Wzc, an integral cytoplasmic membrane tyrosine autokinase protein serves as the master regulator of the biosynthesis and export of many bacterial capsular polysaccharides and exopolysaccharides. Wzc comprises a large periplasmic domain, two transmembrane helices and a C-terminal cytoplasmic kinase domain with a tyrosine-rich tail. Wzc regulates polymerisation functions through cycling the formation and dissociation of an octameric complex, driven by changes in the phosphorylation status of the tyrosine-rich tail. E. coli Wzc serves a model for a wider family of polysaccharide co-polymerases.

Here, we report the characterisation of the structures WzcK540M2YE (Y718E, Y717E), WzcK540M3YE (Y718E, Y717E and Y715E) and WzcK540M3YE_N711Y (an additional N711Y mutation) corresponding to different phosphorylation states. When Y715 occupies the active site (1pY), Y713 is bound in the same pocket. The structural and MD data reported here confirm this hypothesis, showing that the tyrosine most stably positioned at the active site is the one immediately N-terminal to the phosphotyrosine (or the engineered Tyr-to-Glu mutation). We show that it is binding of the i-2 tyrosine to the tyrosine pocket (where i is the number of the residue positioned at the kinase active site) orders the tail between the tyrosine at the active site and helix α23. The presence of the negatively charged E675 in the tyrosine pocket we suggest is incompatible with binding a negatively charged phosphorylated tyrosine (or glutamic acid side chain). During the progressive phosphorylation sequence, the kinase domain is a rigid body. Structural alignment of the kinase domains of monomers of the full-length protein reveals increasing tilting of the transmembrane and periplasmic regions. When the octamer is viewed from the periplasm to the cytoplasm, progressive phosphorylation results in a clockwise rotation of transmembrane and periplasmic regions relative to the kinase ring. The movement of helix α1 is directly transmitted to transmembrane helix α2 and then to the periplasmic domain and, in this way, the phosphorylation signal from the cytoplasm is coupled to the periplasm.

>[8x]MTSVTSKQSTILGSDEIDLGRVIGELIDHRKLIISITSVFTLFAILYALLATPIYETDALIQIEQKQGNAILSSLSQVLPDGQPQSAPETALLQSRMILGKTIDDLNLQIQIEQKYFPVIGRGLARLMGEKPGNIDITRLYLPDSDDISNNTPSIILTVKDKENYSINSDGIQLNGVVGTLLNEKGISLLVNEIDAKPGDQFVITQLPRLKAISDLLKSFSVADLGKDTGMLTLTLTGDNPKRISHILDSISQNYLAQNIARQAAQDAKSLEFLNQQLPKVRAELDSAEDKLNAYRKQKDSVDLNMEAKSVLDQIVNVDNQLNELTFREAEVSQLYTKEHPTYKALMEKRQTLQEEKSKLNKRVSSMPSTQQEVLRLSRDVESGRAVYLQLLNRQQELNIAKSSAIGNVRIIDNAVTDPNPVRPKKTIIIVIGVVLGLIVSVVLVLFQVFLRRGIESPEQLEEIGINVYASIPISEWLTKNARQSGKVRKNQSDTLLAVGNPADLAVEAIRGLRTSLHFAMMEAKNNVLMISGASPSAGMTFISSNLAATIAITGKKVLFIDADLRKGYAHKMFGHKNDKGLSEFLSGQAAAEMIIDKVEGGGFDYIGRGQIPPNPAELLMHPRFEQLLNWASQNYDLIIIDTPPILAVTDAAIIGRYAGTCLLVARFEKNTVKEIDVSMKRFEQSGVVVKGCILNGVVKKASSYYRYGHNHYGYSEEDKKHHHHHH> MASGFSFGTAAASTTTLNPTAAAPFSFGATPAASNTGTTGGLGFGAFNAAATPATTTATTGLGGGLFGAKPAAGFTLGGANTATATTTAASTGFSVGFNKPAGSATPFSLPVTSTSSGGLSLASALTSTPATGPSPFTLNLGSTPATTTAAATGLSLGGTLTGLGGSLFQNTNPSATGLGQSTLGQSTLGQSTLGQSLLGQSLLGQSLLGQSTLGQSTLGQSLLGQSLLGLGLNLGAVAPVSQVTTHEGLGGLDFSSSSDKKSDKAGTRPEDSKALKDENLPQLLCQDVENFQKFVKEQKQVQEEISRMSSKAMLKVQEDIKALKQLLSVASSGLQRNALAIDKLKIETAEELKNAEIALRTQKTPPGLQHENTAPADYFHTLVQQFEVQLQQ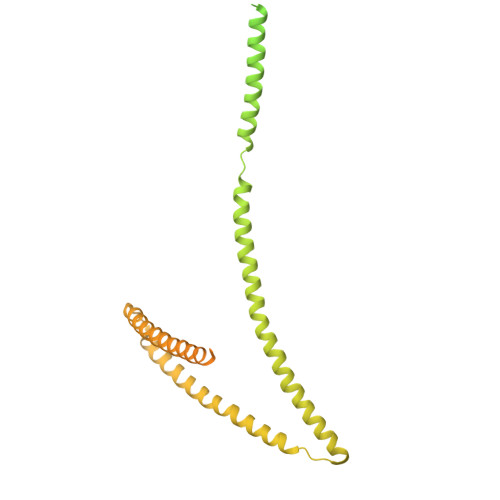YRQQIEELENHLATQSNTLHLSPQDLSMAMQKLYQTFVALAAQLQAVNENFKMLKEQYLGYRKAFLGDSTDVFEARRAEAKKWQNAPRVTTGPTPFSNIPNAAAVAMAATLTQQQQPTTGFGSSSAFGGNTSGSSSFGFGTANKPSGSLSAGFGSTSTSGFNFSNPGINASAGLTFGVSNPSSTSFGTGQLLQLKKPPAGNKRGKR[6-chloranyl-4-[(5-cyclopropyl-1H-pyrazol-3-yl)amino]quinazolin-2-yl]-[(3R)-3-methylpiperazin-1-yl]methanone | C20 H22 Cl N7 O | 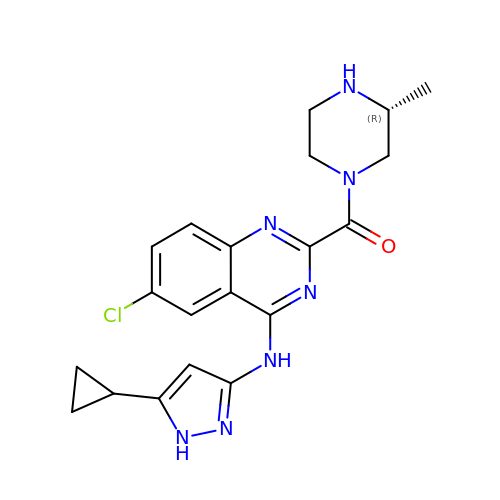RTGFZUPLFGBDKE-LLVKDONJSA-N>[2x]GSHEAVRPLLPDSDSEQPDPVDAQRLDMARRRADANAAPQPGISGRAPAFVHVIAFDLAEPARAEP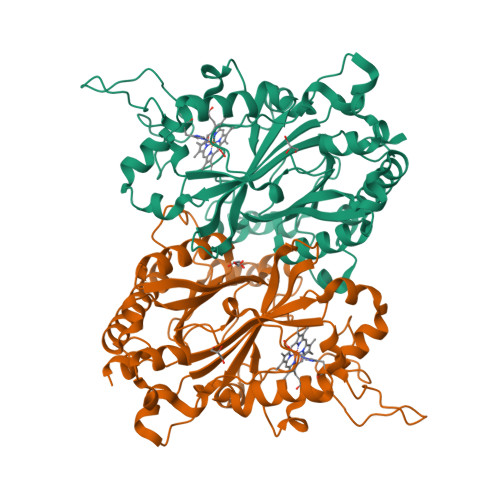AAAREGAATALRTWAEHAARLHADGPEGAASAGLLPASLMVTIGIGGSLLEAMDAADRRPDALADLPEFATDDLRPRWCGGDLMLQVGAEDPMVLAAAVDELVAATAPTTTVRWSLRGFRRTAAAAQDPDATPRNLMGQIDGTANPAQDHPLFTRTVTAPPADDPAHAWMDGGSYLVVRRIRMLLDEWRRLDVPDRERVIGRHLDTGAPLGGEKETDPVVLTARDADGRLVIPEDAHVRLANPENNLGARMVRRGYNYDEGWRDDGVRDAGLLFMAWQGNPATGFVPVQRSLVEQGDALNRYTRHEGSALFAVPAATADRYPGQDLVEG> GAMDHVEFGSGDPGSEIIESVPPAGPEASESTTDENEDDIQFV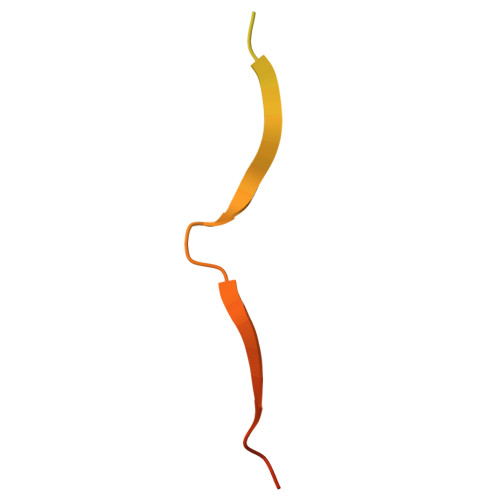SEGPLRPVLEYIDLVSSDDEEP CMY-185 is a CMY-2-like β-lactamase and was identified in an Escherichia coli clinical strain isolated from a patient who underwent treatment with ceftazidime-avibactam. CMY-185, possessing four amino acid substitutions of A114E, Q120K, V211S, and N346Y relative to CMY-2, confers high-level ceftazidime-avibactam resistance, and accumulation of the substitutions incrementally enhances the level of resistance to this agent. The substituted Y346 residue is a major driver of the functional evolution as it rejects primary avibactam binding due to the steric hindrance and augments oxyimino-cephalosporin hydrolysis through a drastic structural change, rotating the side chain of Y346 and then disrupting the H-10 helix structure. The other substituted residues E114 and K120 incrementally contribute to rejection of avibactam inhibition, while S211 stimulates the turnover rate of the oxyimino-cephalosporin hydrolysis.

To obtain further structural insights on CMY-185, we determined the crystal structures of the CMY-185 free form and its complex with ceftazidime at the resolution of 1.35 and 2.40 Å, respectively. Structural comparison with these enzymes showed that the CMY-185 free-form structure is quite similar to the structure of CMY-2 and CMY-136 with the root-mean-square deviation (RMSD) values of 0.45 and 0.52 Å, respectively. The substituted residues K120, S211, and Y346 in CMY-185 are located adjacent to the substrate binding site. The residues S211 and Y346 form hydrogen bonds with residues E61 and S318, respectively, while the side chain of K120 is exposed to the bulk solvent. The substituted residue E114 is located at the inner molecule, and it forms hydrogen bonds with the main chain nitrogen atoms of G116 and L117. The effect of the A114E substitution to the overall structure appears to be minimal, resulting in the loop structure around the P118 residue pushed up ~1 Å away. Structural studies indicated that the A114E substitution did not alter the overall structure, and it instead seemed to enhance the intramolecular interaction through the hydrogen bond formation compared to alanine.

>[2x]MKTEQQIADIVNRTITPLMQEQAIPGMAVAVIYQGKPYYFTWGKADIANNHPVTQQTLFELGSVSKTFNGVLGGDAIARGEIKLSDPVTKYWPELTGKQWQGIRLLHLATYTEGGLPLKIPDDVRDKAALLHFYQNWQPQWTPGAKRLYANSSIGLFGALAVKPSGMSYEEAMTRRVLQPLKLAHTWITVPQNEQKDYAWGYREGKPVHSSPGQLDAEAYGVKSSVIDMARWVQANMDASHVQEKTLQQGIALAQSRYWRIGDMYQGLGWEMLNWPLKADSIINGSDSKVALAALPAVEVNPPAPAVKASWVHKTGSTGGFGSYVAFVPEKNLGIVMLANKSYPYPVRVEAAWRILEKLQ> GSHMFDYMFKILIIG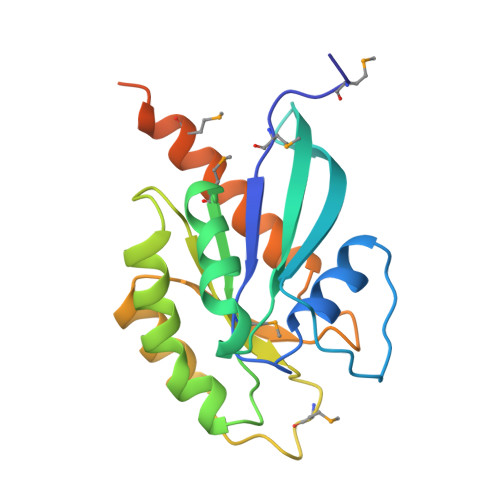NSSVGKTSFLFRYADDSFTPAFVSTVGIDFKVKTIYRNDKRIKLQIWDTAGLERYRTITTAYYRGAMGFILMYDITNEESFNAVQDWSTQIKTYSWDNAQVLLVGNKCDMEDERVVSSERGRQLADHLGFEFFEASAKDNINVKQTFERLVDVICEKMSESLDTADPAVTGAKQGPQLTDQQAPPHQD>[14x]AEPVYPDQLRLFSLGQGVCGDKYRPVNREEAQSVKSNIVGMMGQWQISGL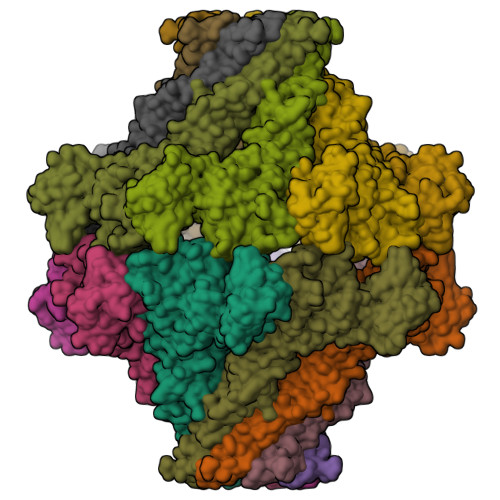ANGWVIMGPGYNGEIKPGTASNTWCYPTNPVTGEIPTLSALDIPDGDEVDVQWRLVHDSANFIKPTSYLAHYLGYAWVGGNHSQYVGEDMDVTRDGDGWVIRGNNDGGCDGYRCGDKTAIKVSNFAYNLDPDSFKHGDVTQSDRQLVKTVVGWAVNDSDTPQSGYDVTLRGDTATNWSKTNTYGLSEKVTTKNKFKWPLVGETELSIEIAANQSWASQNGGSTTTSLSQSVRPTVPARSKIPVKIELYKADISYPYEFKADVSYDLTLSGFLRWGGNAWYTHPDNRPNWNHTFVIGPYKDKASSIRYQWDKRYIPGEVKWWDWNWTIQQNGLSTMQNNLARVLRPVRAGITGDFSAESQFAGNIEIGAPVPLAADSKVRRARSVDGAGQGLRLEIPLDAQELSGLGFNNVSLSVTPAANQLEHHHHHH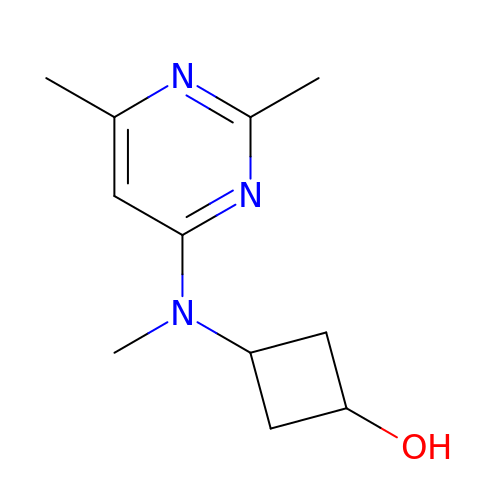trans-3-[(2,6-dimethylpyrimidin-4-yl)(methyl)amino]cyclobutan-1-ol | C11 H17 N3 O | SEZOHQAJJCEOMQ-MGCOHNPYSA-N> SAPVSIWSRVVQFGTGWGFWVSGHVFITAKHVAPPKGTEIFGRKPGDFTVTSSGDFLKYYFTS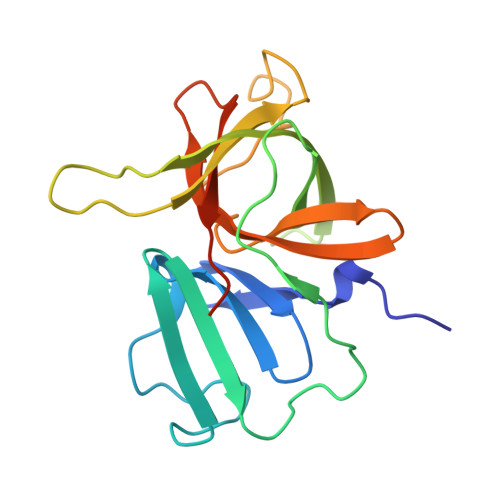AVRPDIPAMVLENGCQEGVVASVLVKRASGEMLALAVRMGSQAAIKIGSAVVHGQTGMLLTGSNAKAQDLGTIPGDAGCPYVYKKGNTWVVIGVHVAATRSGNTVIAATHGEPTLEALEFQG> MTTPTPTQVWRATVPELPPLVDEAGDTGSATARAADTAERLLLLLHYSIDWESSWVADPKHRKTYWDELLPGRVR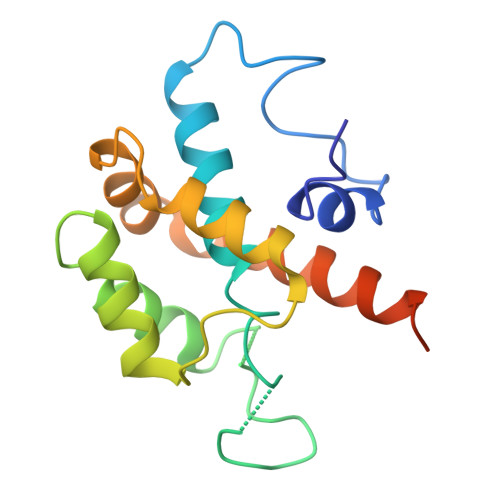RAAYRADTLDRWWSEVAGQLGAPAPRHRDRRLELATLLREPALPVITVLRDSLPALLLRVRIIAEAVAAQRGNNSAATSSADPNEPA> ANGNEGLSTTTKYIFVPIATIGCGKTTVFNTLNNLFPQWTHIQNDNISKKAKLKICDLTLLALEDDDQSVVLFDRNNSASRERRQIFTTIDQKRDEHLDDTVDLKYIAINFIPEDLSEEELWDITYNRVIQRGDNHQSIKSQLDENLVESVMKGFIQRYQPINTSRSPDDQFDHVIHLKLSKDENSLKSSLENVRIIIDDLVQNFPDLIKEKPADELINECFQKALDYKPTFVKNMTANTIKKDPTYYGIAMHYSSILENLEIVSHNEHFQNIKSHIQTEFHVTLGHIASSKQDKAGRVKWKKLVKTLGKGDPNKPKSALKFFADVKLLQIVINTDKLACIKVEILKIYDTNDVLQ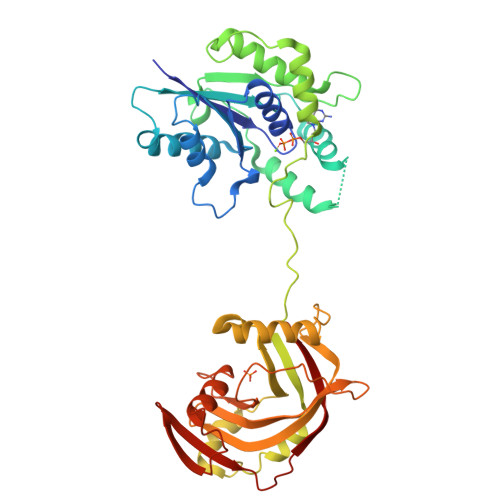SEIEPINKQLHITIGCIPPATAVESNITLEELYDNPDEQELKPDGTYKCGDDTLHVFNFDNPDLKLFSQQLFVAYQ>[2x]AMPL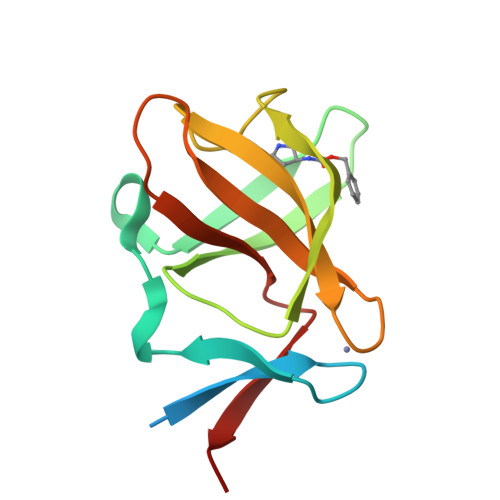DAGGQNSTQMVLAPGASIFRCRQCGQTISRRDWLLPMGGDHEHVVFNPAGMIFRVWCFSLAQGLRLIGAPSGEFSWFKGYDWTIALCGQCGSHLGWHYEGGSQPQTFFGLIKDRLAEGPAD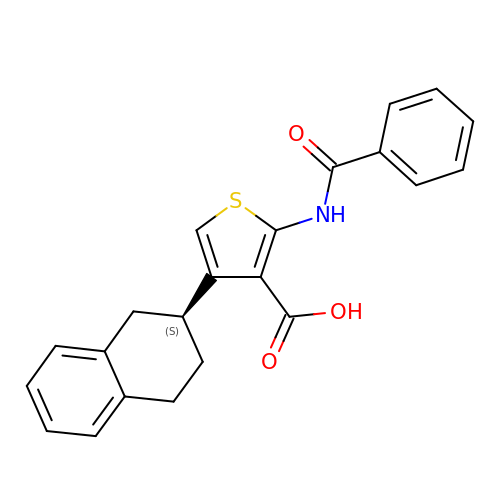2-benzamido-4-[(2~{S})-1,2,3,4-tetrahydronaphthalen-2-yl]thiophene-3-carboxylic acid | C22 H19 N O3 S | ITAWNUSVGMPVHR-KRWDZBQOSA-N>MIILGYNGFSQIAELFGRLYGYTADSVDRHSFLGHDAAAALFVDGELVAAVEEERMNRQKKTTAFPANAMRWCLEQAGISYEDVDYYAFGWNFTAEFADAAITGLASAPIPPEYKFQAIGSFGELWNGALGRTALIEDFTRHTGYALPDEKLITVPHHRAHLACGRTFSGLGDAAFLINDGQAEADSAIMGEVRDGKVEVFERFTIDAKNSLAQLFANITRYLGFTPNNDEYKVMGLAGFGKAPDEQDNPLLTKVVTLEEGGRYSLALANDPRGPRAYDPLFDELFDGNDDNRQEFDFRVRVACAAQQVIEAVTAHQLRALAEATELRDLIFEGGLALNCVNNTKLLEELPFTRVEVSFGASDPGVSIGAAAHVAREKSVALTPTESPYLGPEFGEDEIRATLEEYTSSVTWEQLPSDEVVGKTAELLTGKTVIGWFQGRTEYGPRALGNRSILANPSYADMKDVINNRVKHREPFRPFAPIVLEENAARVFEMGRKERSPYMTFVFPVRPEYTEKIAAATHVDATSRIQTVTEDSNPRLAALLREFTSRTDVPCLVNTSFNVA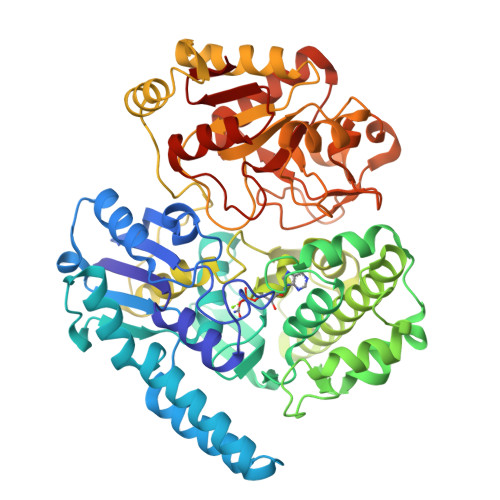GEPIVCSPKDAVECFLGTDIDHLVIGDFLVSKR[4x]>[6x]MREVVIVDSVRTGLAKSFRGKFNLTRPDDMAAHCVDALLARNDLDPLLVDDCIVGAGSNEGAQGHNIGRNVAVLSGLGIQVPGMTLNRYCSSGLQAIAIAANQIASGCSEVIVAGGVESITLTLKSVNTDHLVNPLLQREVPGIYYPMGQTA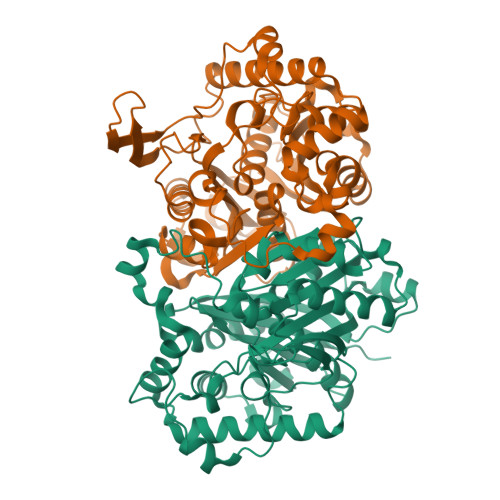EIVARRYGITREAQDAYALQSQQRMARAQADGLFADEIVPMTTRYAVEDKASGEKQVLDGVVDRDDCNRPDTTLEGLASLKPAFAEDGSVTAGNASQLSDGASMTLLMSLEKALALGLEPKAFFRGFTVAGCEPDEMGIGPVFSVPKLLKAKGLKIADVDLWELNEAFASQCLYCRDRLEIDNEKYNVNGGSIAIGHPFGMTGSRQVGHLVRELHRRNLRYGVVTMCVGGGMGASGLFEAVRLEHHHHHH>MSKKEVCSVAFLKAVFAE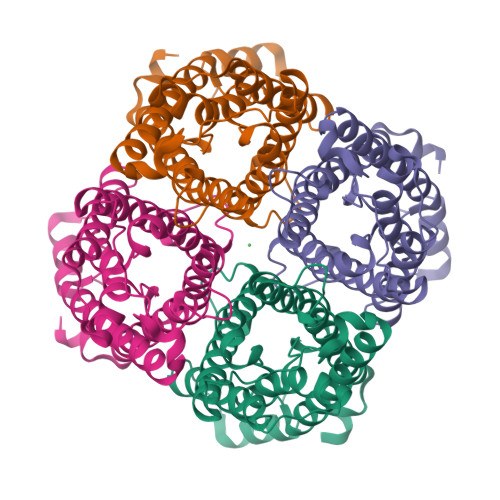FLATLIFVFFGLGSALKWPSALPHILQIALAFGLAIGTLAQALGPVSGGHINPAITLALLVGNQISLLRAFFYVAAQLVGAIAGAGILYGVAPLNARGNLAVNALNNNTTQGQAMVVELILTFQLALCIFASTDSRRTSPVGSPALSIGLSVTLGHLVGIYFTGCSMNPARSFGPAVVMNRFSPAHWVFWVGPIVGAVLAAILYFYLLFPNSLSLSERVAIIKGTYEPDEDWEEQREERKKTMELTTR[4x]>[5x]MVVDGDLHIHSHYSKAVSKLMTFPIIAENAKLKGLNLVGTGDSLNPHWEKELLKHSKPIDDGTFEVNGVKFILTCEVEDKRRVHHLLIFPTLSQVREFREKVKIYSTNIESEGRPNLNLTAEEIAEMANELDILIGPAHAFTPWTSLYKEYDSLKDAYGDAKIDFLELGLSADSDMADMIKAHHSIPYLSNSDAHSPNPHRLGREFNRFEVKDVTFEEIRKAIKGVGGRKIM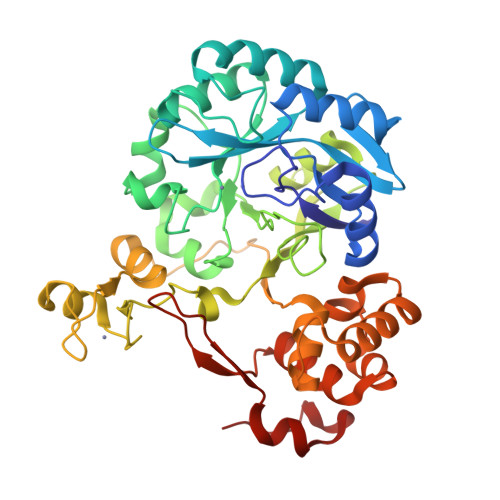LNAGLDPRLGKYHLTACSRCYTKYTLQDAVSLSWKCPKCGGIIKKGVRDRILELADTSEKPKDRPPYVRLAPLAEIIAMVLGKGIESKAVKLLWNRFLREFGSEIRVLIDLPIESIASVHEGVAKAIWAYRNNKLIIVPGGGGKYGEIRIPEEILKAKIEDLNSIEIS>LPTDTTTFKRIFLKRMPSIRESLKERGVDMARLGPEWSQPMKRLTLGNTTSSVILTNYMDTQYYGEIGIGTPPQTFKVVFDTGSSNVWVPSSKCSRLYTACVYHKLFDASDSSSYKHNGTELTLRYSTGTVSGFLSQDIITVGGITVTQMFGEVTEMPALPFMLAEFDGVVGMGFIEQAIGRVTPIFDNIISQGVLKEDVFSFYYNRDSENSQSLGGQIVLGGSDPQHYEGNFHYINLIKTGVWQIQMKGVSVGSSTLLCEDGCLALVDTGASYISGSTSSIEKLMEALGAKKRLFDYVVKCNEGPTLPDISFHLGGKEYTLTSADYVFQESYSSKKLCTLAIHAMDIPPPTGPTWALGATFIRKFYTEFDRRNNRIGFALAR[4x];>[4x]DRVYIHPFHLVIHNESTCEQLAKANAGKPKDPTFIPAPIQAKTSPVNEKALQDQLVLVAAKLDTEDKLRAAMVGMLANFLGFRIYGMHSELWGVVHGATVLSPTAVFGTLASLYLGALDHTADRLQAILGVPWKDKNCTSRLDAHKVLSALQAVQGLLVAQGRADSQAQLLLSTVVGVFTAPGLHLKQPFVQGLALYTPVVLPRSLDFTELDVAAEKIDRFMQAVT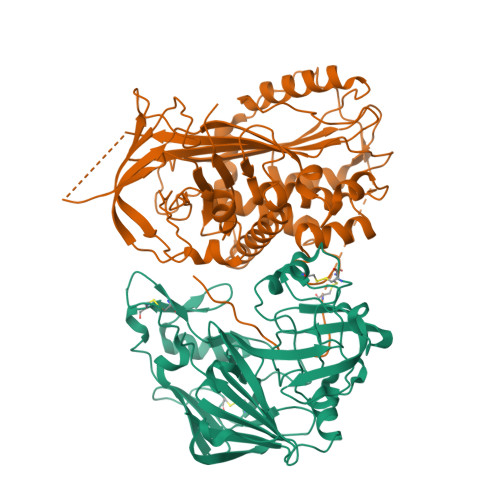GWKTGCSLMGASVDSTLAFNTYVHFQGKMKGFSLLAEPQEFWVDNSTSVSVPMLSGMGTFQHWSDIQDNFSVTQVPFTESACLLLIQPHYASDLDKVEGLTFQQNSLNWMKKLSPRTIHLTMPQLVLQGSYDLQDLLAQAELPAILHTELNLQKLSNDRIRVGEVLNSIFFELEADEREPTESTQQLNKPEVLEVTLNRPFLFAVYDQSATALHFLGRVANPLSTA N-CYCLOPENTYL-2-[4-(TRIFLUOROMETHYL)PHENYL]-3H-IMIDAZO[4,5-B]PYRIDINE-7-SULFONAMIDE | C18 H17 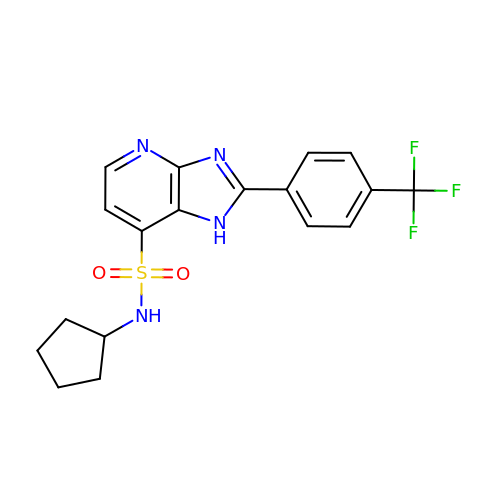F3 N4 O2 S | JBHHWVFQIGPHPU-UHFFFAOYSA-N>MSLIYQIAKEFDFCYGHRVWSQELNPDFSLDPCLSCRHLHGHQGKVIVHLESRELQRGMVTDFAHLNWFKRF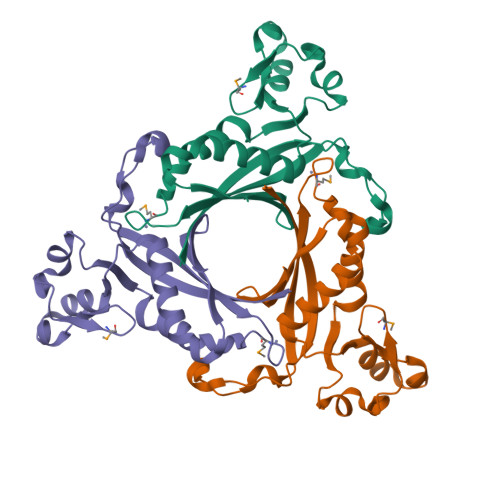IDEVLDHRFIIDIDDPLFPTLLPHFADKSALVWMEEGYARVDFERIKGESSPILELYESFVVVRFVPTSESIASWLLELLRSRIQPLGVKVSSVEFLETPKSRARVYNEGHHHHHH[6x]> MKEYTLDKAHTDVGFKIKHLQISNVKGNFKDYSAVIDFDPASAEFKKLDVTIKIASVNTENQTRDNHLQQDDFFKAKKYPDMTFTMKKYEKIDNEKGKMTGTLTIAGVSKDIVLDAEIGGVAKGKDGKEKIGFSLNGKIKRSDFKFATSTSTITLSDDINLNIEVE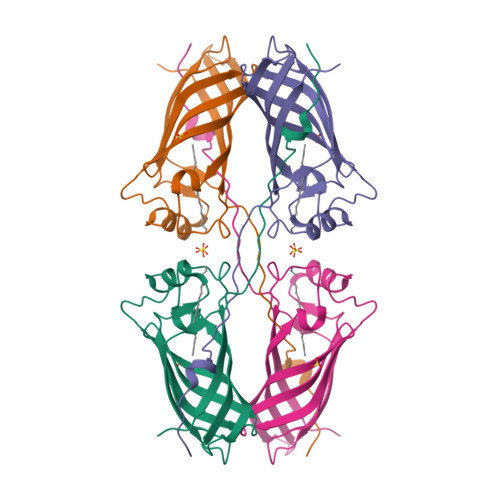ANEKEGGSHHHHHH> GHMPLLSASIVSAPVVTSETYVDIPGLYLDVAKAGIRDGKLQVILNVPTPYATGNNFPGIYFAIATNQGVVADGCFTYSSKVPESTGRMPFTLVATIDVGSGVT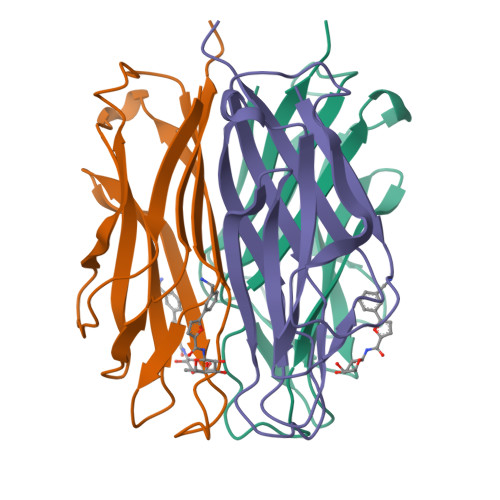FVKGQWKSVRGSAMHIDSYASLSAIWGTAA>[2x]KFNDTLFG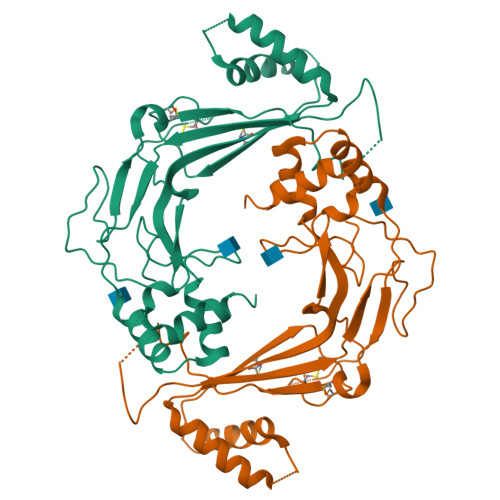EMLHGYNNRTQHVNQGQVFQMTFRENNFIKDFPQLADGLLVIPLPVEEQCRGVLSEPLPDLQLLTGDIRYDEAMGYPMVQQWRVRSNLYRVKLSTITLAAGFTNVLKILTKESSREELLSFIQHYGSHYIAEALYGSELTCIIHFPSKKVQQQLWLQYQKETTELGSKKELKSMPFITYLSGLLTAQMLSDDQLISGVEIRCEEKGRCPSTCHLCRRPGKEQLSPTPVLLEINRVVPLYTLIQDNGTKEAFKSALMSS> MKLPLLLALLFGAVSALHLRSETSTFETPLGAKTLPEDEETPEQEMEETPCRELEEEEEWGSGSEDASKKDGAVESISVPDMVDKNLTCPEEEDTVKVVGIPGCQTCRYLLVRSLQTFSQAWFTCRRCYRGNLVSIHNFNINYRIQCSVSALNQGQVWIGGRITGSGRCRRFQWVDGSRWNFAYWAA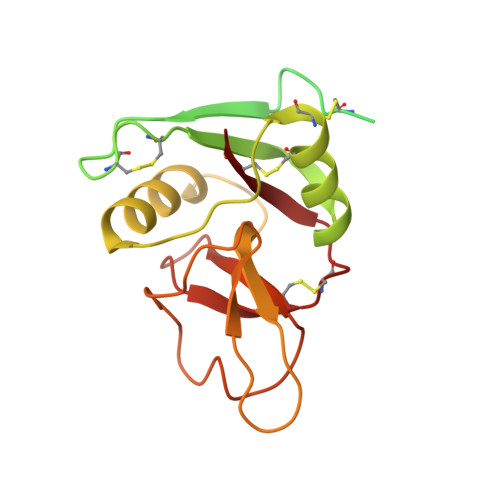HQPWSRGGHCVALCTRGGHWRRAHCLRRLPFICSY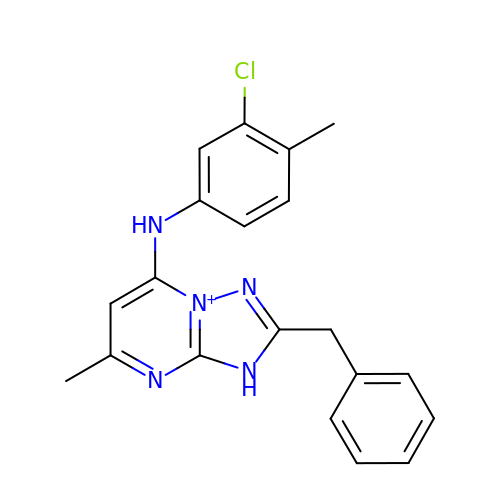2-benzyl-7-[(3-chloro-4-methylphenyl)amino]-5-methyl-3H-[1,2,4]triazolo[1,5-a]pyrimidin-8-ium | C20 H19 Cl N5 | QGHMESXINCFELP-UHFFFAOYSA-O3-chloro-N-(5-chloro-2-methyl-1,3-benzothiazol-6-yl)-2-hydroxybenzene-1-sulfonamide | C14 H10 Cl2 N2 O3 S2 | 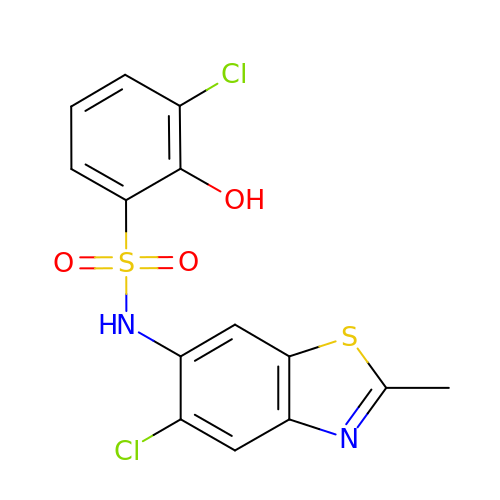DGNXLFRZMYASGW-UHFFFAOYSA-N> MKPPRPVRTCSKVLVLLSLLAIHQTTTAEKNGIDIYSLTVDSRVSSRFAHTVVTSRVVNRANTVQEATFQMELPKKAFITNFSMIIDGMTYPGIIKEKAEAQAQYSAAVAKGKSAGLVKATGRNMEQFQVSVSVAPNAKITFELVYEELLKRRLGVYELLLKVRPQQLVKHLQMDIHIFEPQGISFLETESTFMTNQLVDALTTWQNKTKAHIRFKPTLSQQQKSPEQQETVLDGNLIIRYDVDRAISGGSIQIENGYFVHYFAPEGLTTMPKNVVFVIDKSGSMSGRKIQQTREALIKILDDLSPRDQFNLIVFSTEATQWRPSLVPASAENVNKARSFAAGIQALGGTNINDAMLMAVQLLDSSNQEERLPEGSVSLIILLTDGDPTVGETNPRSIQNNVREAVSGRYSLFCLGFGFDVSYAFLEKLALDNGGLARRIHEDSDSALQLQDFYQEVANPLLTAVTFEYPSNAVEEVTQNNFRLLFKGSEMVVAGKLQDRGPDVLTATVSGKLPTQNITFQTESSVAEQEAEFQSPKYIFHNFMERLWAYLTIQQLLEQTVSASDADQQALRNQALNLSLAYSFVTPLTSMVVTKPDDQEQSQVAEKPMEGESRNRNVHSGSTFFKYYLQGAKIPKPEASFSPRRGWNRQAGAAGSRMNFRPGVLSSRQLGLPGPPDVPDHAAYHPFRRLAILPASAPPATSNPDPAVSRVMNMKIEETTMTTQTPAPIQAPSAILPLPGQSVERLCVDPRHRQGPVNLLSDPEQGVEVTGQYEREKAGFSWIEVTFKNPLVWVHASPEHVVVTRNRRSSAYKWKETLFSVMPGLKMTMDKTGL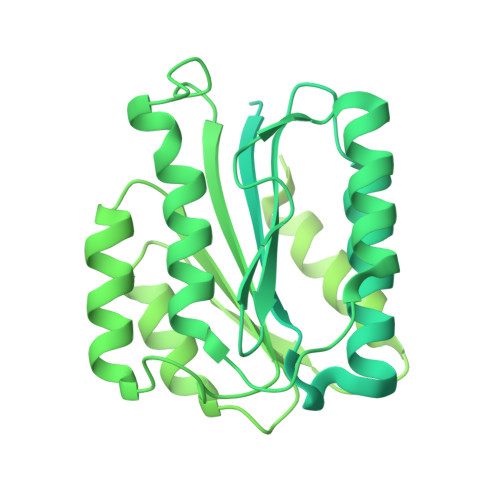LLLSDPDKVTIGLLFWDGRGEGLRLLLRDTDRFSSHVGGTLGQFYQEVLWGSPAASDDGRRTLRVQGNDHSATRERRLDYQEGPPGVEISCWSVEL> MSKAMALRRLMKEYKELTENGPDGITAGPSNEDDFFTWDCLIQGPDGTPFEGGLYP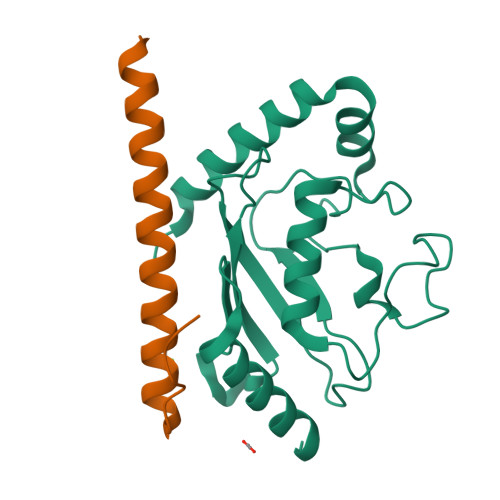ATLKFPSDYPLGPPTLKFECEFFHPNVYKDGTVCISILHAPGDDPNMYESSSERWSPVQSVEKILLSVMSMLAEPNDESGANIDACKMWREDREEYCRVVRRLARKTLGLLVPR;> GSHMLSSRISSSDNSSSSTGNEEVRNRSKLPSSKKEREELFRKRKEEMILAARKRMEGKIKGEKQDKN>MTWPDVPIAAAPGISYFTPAQSPPAGTARNPQTSGKAIPKLFQPLTIRGHTFQNRLGVAPMCQYSADDGHLTPWHMAHYGGIAQRGPGMIIIEATGVVPEGRITPGCVGLWKDSQIAPLKQVVEFAHSQGQKIGIQLAHAGRKASTVPPWLGGVTATNAVGGWTENVKGPSAIPFAEGEIVPKAMTKEDIEEVKTAWVAAVERAVAAGVDFIEIHNAHGYLLSSFLSPSSNQRTDDYGGSFENRIRLSLEISQLTRDTVGPNMPVFLRVSATDWLEKSMPEEKGWKLEDTVEFSRALAAQGAIDLIDISTGGVHAAQKVTSGVGFQVPFAKAVKEAVGQKMLVSAVGTINSGNLAEKILNEDDVDVILVGRAFQRDSGLAWAFAKDLDVEIAMAGQIRWGFTSFRNASEYIQPNSMKASIFD[8x]

Ene‐reductases (ERs) catalyze the asymmetric reduction of C=C double bonds in α,β‐unsaturated compounds, where the double bond is conjugated to an electron‐withdrawing group (EWG), such as a carbonyl moiety. The mechanism can be dissected into two half‐reactions, the first half‐reaction (reductive half‐reaction) begins with the transfer of a hydride from NAD(P)H to the ER‐bound flavin cofactor, FMN. In the next half‐reaction (oxidative half‐reaction), the reduced flavin transfers a hydride ion to the β‐carbon (the carbon next to the EWG). This is accompanied by a proton transfer to the substrate coming from a tyrosine residue in the active site, being transferred to the α‐carbon.

PsOYE2 crystallized in the monoclinic space group P21 with four dimers in the asymmetric unit. The crystal structure was determined at a resolution of 2.3 Å. DLS analysis and size exclusion chromatography already suggested that PsOYE2 forms dimers in solution, with estimated molecular weights of 68 kDa and 78 kDa, respectively. The ER fold consists of eight twisted β‐strands surrounded by eight α‐helices, [(β/α)8] or TIM‐barrel structure, as predicted previously using Alphafold2 and in alignment with other Class III enzymes. A substantial portion of the N‐terminus (44 residues) interacts with the neighboring protomer, creating a tightly bound dimer, which might be a characteristic of fungal enzymes. The C‐terminal region is also involved in dimer formation and shapes the FMN binding pocket of the other monomer. The FMN cofactor, situated on the C‐terminal side of the barrel, has interactions through the phosphate group with the side chain of Arg371 and backbone nitrogen atoms of Arg371, Gly370 and Thr348 (of the adjacent protomer). The ribityl part is stabilized by Arg368, and the isoalloxazine on the re face via hydrophobic contacts with Pro60 and Met61, and the backbone carbonyl atom of Pro60 to N5 and N10. The “arginine finger”, a distinctive characteristic of Class III ERs, was observed in PsOYE2 being represented by Arg371. In place of Arg in comparison to YqjM, PsOYE2 exhibited a Trp, which participates in the substrate binding site and might contribute to form a large hydrophobic substrate site, along with Phe, another residue believed to play a role at the same site.> GWSTELEK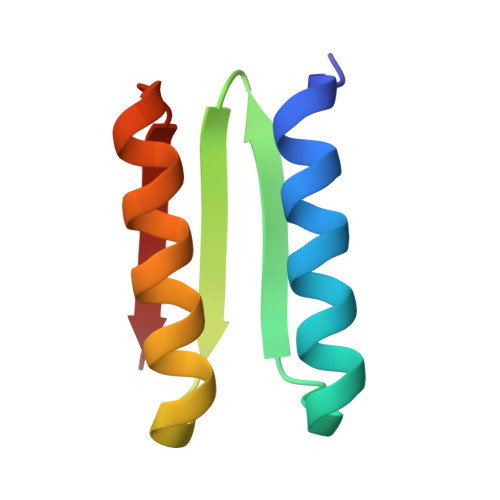HREELKEFLKKEGITNVEIRIDNGRLEVRVEGGTERLKRFLEELRQKLEKKGYTVDIKIE> AQDDSTPDSLFAGLVGEYYGTNSQLNNISDFRALVDSKEADATFEAANISYGRGSSDVAKGTHLQEFLGSDASTLSTDPGDNTDGGIYLQGYVYLEAGTYNFKVTADDGYEITINGNPVATVDNNQSVYTVTHASFTISESGYQAIDMIWWDQGGDYVFQPTLSADGGSTYFVLDSAILSSTGETPYTT

MpPA14 (Marinomonas primoryensis PA14 domain) lectin is a domain of a 1.5-MDa adhesin responsible for a symbiotic bacterium-diatom interaction in Antarctica. Bioinformatic analyses indicated the presence of an ∼20-kDa domain near the C terminus of MpIBP that is a member of the PA14 family, which is a carbohydrate-binding lectin module widely distributed across several kingdoms of life. PA14 domains share a β-sandwich fold and the presence of two consecutive aspartate residues in a cis peptide linkage (DcisD). The DcisD motif coordinates a Ca2+ ion that is directly involved in binding polar vicinal hydroxyl groups of various carbohydrates.

Glucose, GlcNAc, and other glucopyranose-containing carbohydrates, including 2-deoxy-glucose, methyl-α-glucose, and two disaccharides (sucrose and trehalose), all bound to the Mp-PA14-Ca1 via their trans vicinal 3,4-diols (ionic bond length, 2.5 Å) in gauche configuration with a dihedral angle of ∼60°. This interaction is further enhanced with the diol being coordinated by the side chain carboxyl and hydroxyl oxygens of the DcisD motif, and main-chain and side chain protein ligands from L11 (Gln156, Gly157, and Asp159).> GPDSMAGLELLSDQGYRVDGRRAGELRKIQARMGVFAQADGSAYIEQGNTKA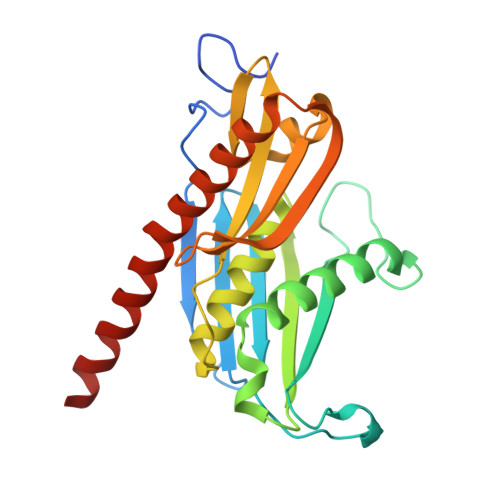LAVVYGPHEIRGSRARALPDRALVNCQYSSATFSTGERKRRPHGDRKSCEMGLQLRQTFEAAILTQLHPRSQIDIYVQVLQADGGTYAACVNAATLAVLDAGIPMRDFVCACSAGFVDGTALADLSHVEEAAGGPQLALALLPASGQIALLEMDARLHEDHLERVLEAAAQAARDVHTLLDRVVRQHVREASILLGD> MDLAKLGLKEVMPTKINLEGLVGDHAFSMEGVGEGNILEGTQEVKISVTKGAPLPFAFDIVSVAFTYGNRAYTGYPEEISDYFLQSFPEGFTYERNIR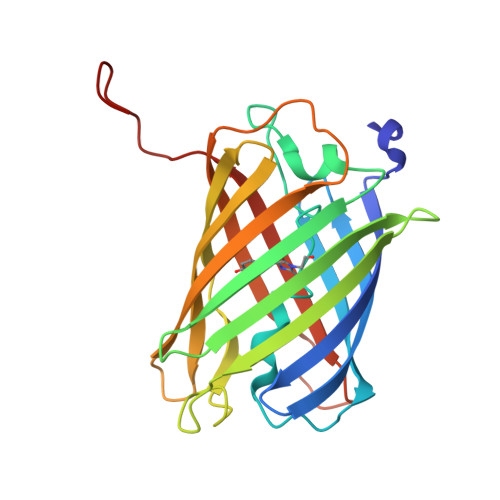YQDGGTAIVKSDISLEDGKFIVNVDFKAKDLRRMGPVMQQDIVGMQPSYESMYTNVTSVIGECIIAFKLQTGKHFTYHMRTVYKSKKPVETMPLYHFIQHRLVKTNVDTASGYVVQHETAIAAHSTIKKIEGSLP>MRPPMYTSTNTEVPSRLVKNEHGSWQLIVNGKPFIMLAGELHNSSASTTEYLNSLWTSLKTLNLNTVLAPIAWEQFEPQEGIFDYTLINNMIDGARKNGFKLSILWFGSWKNGESSYAPTWVKEDTKRFFRVKSVEGKEIETISPFCENAMKADAKAFKTLVEHIKKVDQATGTVIALQPENEVGIFQGMDYSKASLAAYEQE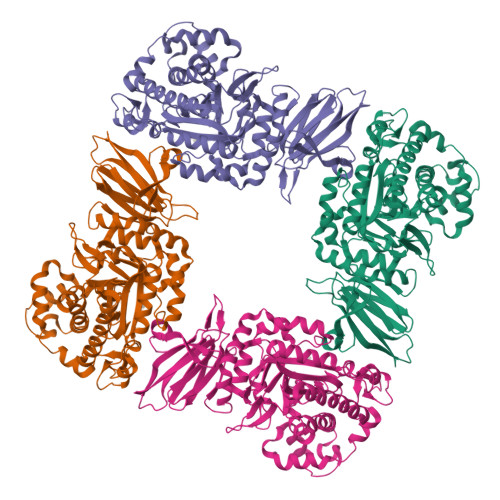VPQALIQYMKKNRKNLRKELLSVWEENGARTSGAWKTVFGDNAWSKSFYTTWQYATYIDFISAGAKEIYPLPTFCNCWLVQKPDDMPGVYPNGGPVSRVMDIWKAAAPHIDVLAPDIYLSDFKNIVADYHRADNPLLIPEAVMKPANAFWAFGEHSALCYSPFGIEDGADNFVFAQSYKVLNELIPLISEHQGSDRMIGVMKMPGESERTVTMGDYQLCIKYDAEDAYGLIIQTGKNEFVVAGINFKVYFTSTDKKKTGYIKQVWEGGYDTDGEWKATRLLNGDETYHNAVLIAKGRRTFTSEKSNNYNADHSDEIFVYSPTSYQAVWSPGIYRVTTYLRLEHHHHHH[4x]> MTKRIASVEKTIRIGFVGSLLFGLLPRIIHLYRQAHPNLRIELYEMGTKAQTEALKEGRIDAGFGRLKISDPAIKRTLLRNERLMVA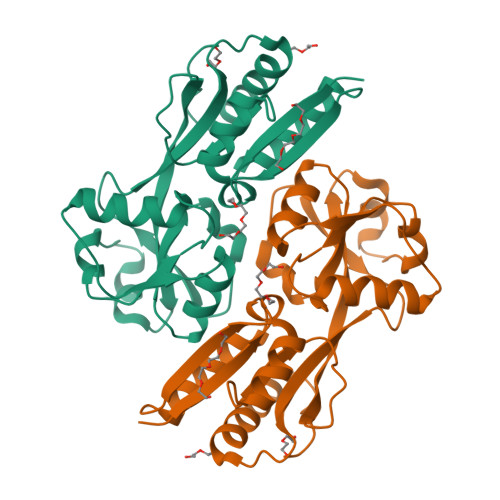VHASHPLNQMKDKGVHLNDLIDEKILLYPSSPKPNFSTHVMNIFSDHGLEPTKINEVREVQLALGLVAAGEGISLVPASTQSIQLFNLSYVPLLDPDAITPIYIAVRNMEESTYIYSLYETIRQIYAYEGFTEPPNWLEHHHHHH>MPRSLANAPIMILNGPNLNLLGQRQPEIYGSDTLADVEALCVKAAAAHGGTVDFRQSNHEGELVDWIHEARLNHCGIVINPAAYSHTSVAILDALNTCDGLPVVEVHISNIHQREPFRHHSYVSQRADGVVAGCGVQGYVFGVERIAALAGAGSARA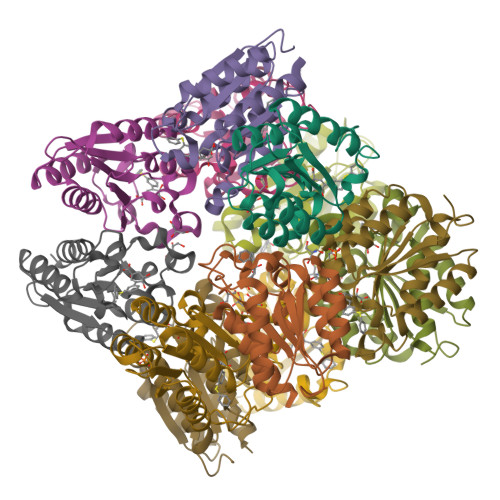[12x]>GSHMASMKKKGSVVIVGRINLSGDTAYAQQTRGEEGCQETSQTGRDKNQVEGEVQIVSTATQTFLATSINGVLWTVYHGAGTRTIASPKGPVTQMYTNVDKDLVGWQAPQGSRSLTPCTCGSSDLYLVTRHADVIPVRRRGDSRGSLLSPRPISYLKGSSGGPLLCPAGHAVGIFRAAVCTRGVAKAVAFIPVES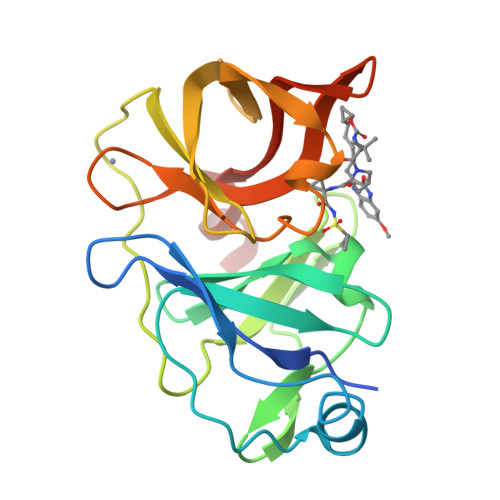LETTMRSP[4x]N-benzyl-2-[(morpholin-4-ylacetyl)amino]-4,5,6,7-tetrahydro-1-benzothiophene-3-carboxamide | C22 H27 N3 O3 S | 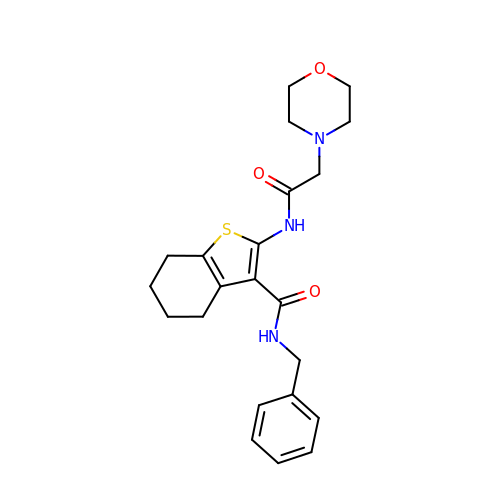JZNVWORYNPPJSO-UHFFFAOYSA-N> MNYNNKILVSESGLSQKHLIHGDEELFQHELKTIFARNWLFLTHDSLIPAPGDYVTAKMGIDEVIVSRQNDGSIRAFLNVCRHRGKTLVSVEAGNAKGFVCSYHGWGFGSNGELQSVPFEKDLYGESLNKKCLGLKEVARVESFHGFIYGCFDQEAPPLMDYLGDAAWYLEPMFKHSGGLELVGPPGKVVIKANWKAPAENFVGDAYHVGWTHASSLRSGESIFSSLAGNAALPPEGAGLQMTSKYGSGMGVLWDGYSGVHSADLVPELMAFGGAKQERLNKEIGDVRARIYRSHLN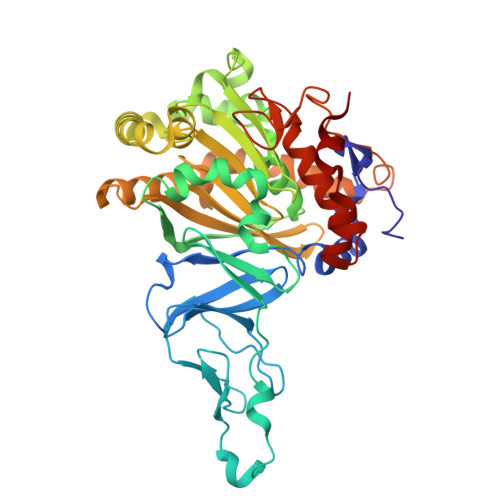CTVFPNNSMLTCSGVFKVWNPIDANTTEVWTYAIVEKDMPEDLKRRLADSVQRTVGPAGFWESDDNDNMETASQNGKKYQSRDSDLLSNLGFGEDVYGDAVYPGVVGKSAIGETSYRGFYRAYQAHVSSSNWAEFEHASSTWHTELTKTTDR We have identified a transporter from Syntrophobacter fumaroxidans (SfMCT) that shares 25 and 27% amino acid sequence identity, and 51 and 57% sequence similarity with the human SLC16 family L-lactate transporters MCT1 and MCT4. In summary, we reported two structures of the bacterial SLC16 homologue SfMCT in complex with the monocarboxylates TSA and L-lactate. We have presented the structures of an L-lactate transporter (SfMCT) with two different bound ligands. Both structures show SfMCT in the pharmacologically relevant outward-open conformation, which is an essential prerequisite for the design of L-lactate transport inhibitors using SfMCT structure-based homology models of human MCT1 and MCT4.

The structure of SfMCT was solved at 2.54 Å resolution by single-wavelength dispersion (SAD) phasing from thiomersal-derivatized crystals. The structure shows SfMCT in an outward-open conformation with a central, conical cavity open to the periplasmic side while the cytoplasmic side of SfMCT is closed. With an average inhibition constant (Ki) of 120 μM, SfMCT has a higher affinity for TSA than for its transported substrate L-lactate (Km = 233 μM). In contrast to L-lactate, TSA is not transported by SfMCT as determined by a micro pH electrode-based transport assay. The carboxylate group of TSA interacts with the hydroxyl group of Y119 (TM4) and the Nη nitrogen atoms of the guanidinium group of R280 (TM8). L145 (TM5) and F335 (TM10) form an ~8 Å wide confinement that accommodates and orients the carboxylate group of TSA for proper binding to Y119 (TM4) and R280 (TM8). The thiol group of TSA is in hydrogen bonding distance to the hydroxyl group of Y331 (TM10) and 3.5 Å from the isobutyl group of L28 (TM1). These two residues trap TSA by partly obstructing the ligand-binding site. The side chains of F359 (TM11) and C362 (TM11) are within a distance of <4 Å from the benzene ring of TSA interacting via hydrophobic interactions.

>MADQQTTMPRWVPLLLGLLGSTTCGMLLYAWSVFIKPLNAEFGWSRAEIAMAFAICCLIFGLMTFPAGRLSDKMGPRKVVMTGGVLLAIGFILSGFIQSKYQLYITYGVIAGFGGGMIYLPPIATAPKWWPDRRALATGFAVVGLGLGSFLMGPLATYIIEKPGMGWRYVFWYCGVAMGIMALIAGAFLEPPPAGWKPAGYTPPAPPAGAAAPKVTRDWTYEEAKGDTKFWLLYLAYFCGSFAGLMVIGHLAGFGRDAGLTAMAAAGAVSSLAFSNAATRILSGWFVDKIGIRVYFAALFALQTAAMIAIFQLGGSVVGLSIVAIVIGWNYGAMFTLFPATCLQFYGPTAQGSNYGLLFTACGLAGFAGPWVGGWLKDTTGTYYLPFLCAAALCALGTAIVFMTKPPEKKHALELEVLFQ[2x]>MSAHRTLLLRLSDSGEPVTSCSYGQGVLTLPSLPLPQGKKLGDMPVYTVKLAIPAGSPVTRDGLIWTNCPPDFSTQFDREKFYKKIIKTSFHEDDHIDLDIYVPGTYCFYLSFKNDKDELETTRKFYFVVLPILSVNDKFIPLNSIAMQSVVSKWMGPTIKDWEKVFARVASKKYNMIHFTPLQHRGESNSPYSIYDQLEFDPTVFKSEKEVADMVERLRTEHNILSLTDIVFNHTANNSQWLLDHPEAGYNHKTSPHLISAIELDKKLLDFSEQMEALGYPVDLKTVDDLIKVMDGIKEHVIGELKLWEFYVVDVKQTVSELREKWGNSKSWSDDNIPSKDDSTNLAQFVRDNATEPGFGSLGERGSNKINIDKFAAILKKLHSEDYNNGIEELATKILNDINLPFYKEYDDDINEVLEQLFNRIKYLRIDDHGPKQGPITKKLPLSEPYFTRFKAKDGEEYALANNGAIWDGNPLVDFASSQSKAYLRREVIVWGDCVKLRYGKGPSDSPYLWERMSKYVEMNARIFNGFRIDNCHSTPLHVGQYFLDVARRVNPNLYVVAELFSGSEAMDCLFVERLGISSLIREAMQAWSEEELSRLVHRHGGRPIGSYKFVPLDDFPYPADVKIDEEYCAYNPDDHSVKCVSEIMIPKTLTATPPHALFMDCTHDNETPNQKRTVEDTLPNAALVAFCSSAIGSVYGYDEVFPQLLDLVQEKRTYSCAENTGISKVKTLLNNMREEIASEAVDIEDSEMHVHHDGQYITFHRTNAKNGKGWYLVARTKFHSSGDQMLPRIKLSQTKATFKAAFSLERTGDAPISDEIIEGIPTKLRELTGFDIGFDENTKETSILLPQDFPQGSIVIFETQQLGIDDSLDHFIRSGAIKATEKLSLESINYVLYRAEQEEYDYSEGRSGAYDIPDYGKPVYCGLQGWVSILRKIIFYNDLAHPLSNNLRNGHWAVDYVVNRLDLYKDKEGVAEVQEWLRSRMERIKQLPSYLVPSFFALVVGIMYGCCRLRAMQLMSDNVGKSTVFVQSLAMTSIQMVSAMKSTSILPDQNIAAMAAGLPHFSTNYMRCWGRDVFISLRGLLLTTGRYEEAKEHILAFAKTLKHGLIPNLLDAGRNPRYNARDAAWFFVQAIQDYVTIVPGGVSLLQEKVTRRFPLD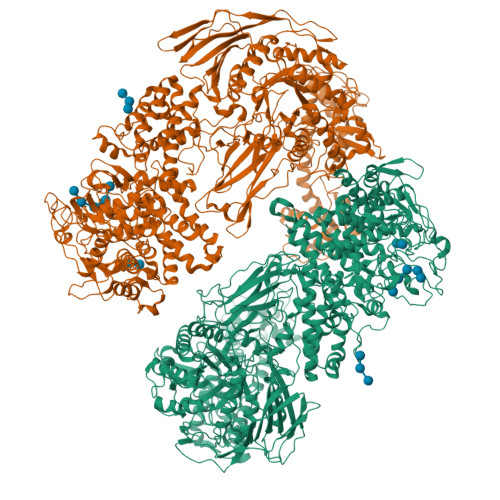DEYIPYDDPKAFSYSSTIEEIIYEILNRHAGGIKYREANAGPNLDRVMKDEGFNVEVNVDWETGLIHGGSQFNCGTWMDKMGESEKANSVGVPGTPRDGAAVEINGLLKSCLRFVLQLSKDGKFKYTEVTKPDGSKISLSSWNDLLQENFERCFYVPKNKEDDNKFEIDATIINRRGIYKDLYRSGKPYEDYQFRPNFTIAMVVAPELFTPDYAAGAIELADQVLRGPVGMRTLDPSDYNYRPYYNNGEDSDDFATSKGRNYHQGPEWVWCYGYFIRAYHYFNFLTNPKCQVEGSAKKLKPSSYLYRKLYSRLLKHREWIENSPWAGLAELTNKDGEVCNDSSPTQAWSTGCLLDLFYDLWISYEELEHHHHHH[2x]> GPLHMGGSPEFPGRLEAADPMSGGLLKALRSDSYVELSQYRDQHFRGDNEEQEKLLKKSCTLYVGNLSFYTTEEQIYELFSKSGDIKKIIMGLDKMKKTACGFCFVEYYSRADAENAMRYINGTRLDDRIIRTDWDAGFKEGRQYGRGRSGGQVRDEYRQDYDAGRGGYGKLAQN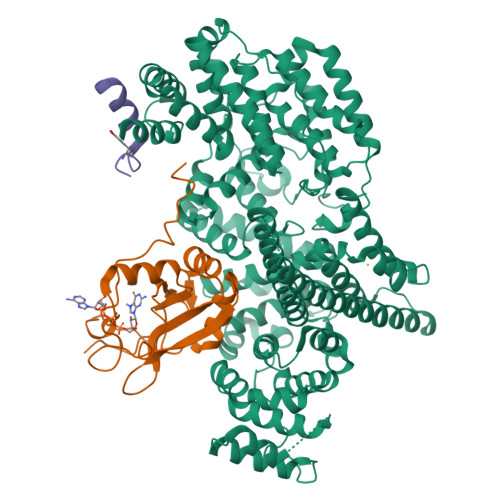Q;> XSEEALPASGKSKYEAMDFDSLLKEAQQSLH;> MANETEDHLESLICKVGEKSACSLESNLEGLAGVLEADLPNYKSKILRLLCTVARLLPEKLTIYTTLVGLLNARNYNFGGEFVEAMIRQLKESLKANNYNEAVYLVRFLSDLVNCHVIAAPSMVAMFENFVSVTQEEDVPQVRRDWYVYAFLSSLPWVGKELYEKKDAEMDRIFANTESYLKRRQKTHVPMLQVWTADKPHPQEEYLDCLWAQIQKLKKDRWQERHILRPYLAFDSILCEALQHNLPPFTPPPHTEDSVYPMPRVIFRMFDYTDDPEGPVMPGSHSVERFVIEENLHCIIKSHWKERKTCAAQLVSYPGKNKIPLNYHIVEVIFAELFQLPAPPHIDVMYTTLLIELCKLQPGSLPQVLAQATEMLYMRLDTMNTTCVDRFINWFSHHLSNFQFRWSWEDWSDCLSQDPESPKPKFVREVLEKCMRLSYHQRILDIVPPTFSALCPVNPTCIYKYGDESSNSLPGHSVALCLAVAFKSKATNDEIFSILKDVPNPNQDDDDDEGFSFNPLKIEVFVQTLLHLAAKSFSHSFSALAKFHEVFKTLAESDEGKLHVLRVMFEVWRNHPQMIAVLVDKMIRTQIVDCAAVANWIFSSELSRDFTRLFVWEILHSTIRKMNKHVLKIQKELEEAKEKLARQHKRRSDDDDRSSDRKDGVLEEQIERLQEKVESAQSEQKNLFLVIFQRFIMILTEHLVRCETDGTSVLTPWYKNCIERLQQIFLQHHQIIQQYMVTLENLLFTAELDPHILAVFQQFCALQAAENLYFQGHHHHHH>[3x]GSHMKTRADLFAFFDAHGVDHKTLDHPPVFRVEEGLEIKAAMPGGHTKNLFLKDAKGQLWLISALGETTIDLKKLHHVIGSGRLSFGPQEMMLET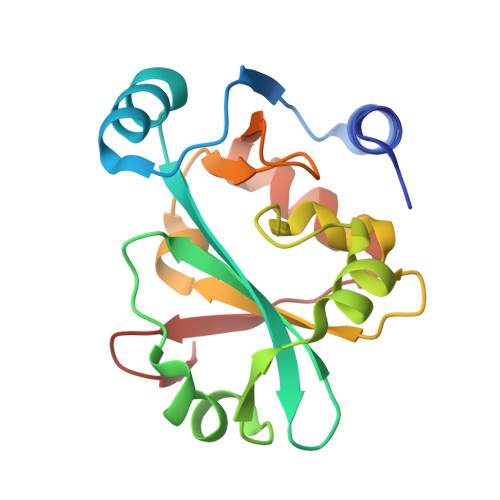LGVTPGSVTAFGLINDTEKRVRFVLDKALADSDPVNFHPLKNDATTAVSQAGLRRFLAALGVEPMIVDFAAMEVVG> MDSTNLNKRPLLQYSLSSLGSQITKWSSSRPTSPVRKARSTENDFLSKQDTSSILPSINDDGGEQWYEKFKPNCLEQVAIHKRKLKDVQEALDAMFLPNAKHRILLLSGPSGCSKSTVIKELSKILVPKYRQNSNGTSFRSTPNEHKVTEFRGDCIVNDLPQMESFSEFLKGARYLVMSNLSLILIEDLPNVFHIDTRRRFQQLILQWLYSSEPLLPPLVICITECEIPENDNNYRKFGIDYTFSAETIMNKEILMHPRLKRIKFNPINSTLLKKHLKFICVQNMKMLKEKNKWNKRQEVIDYIAQETGDIRSAITTLQFWATSSGSLPISTRESTISYFHAIGKVIHGSHSTNNDNEMINNLFENSNNLLSKEDFKLGILENYNTFNKGE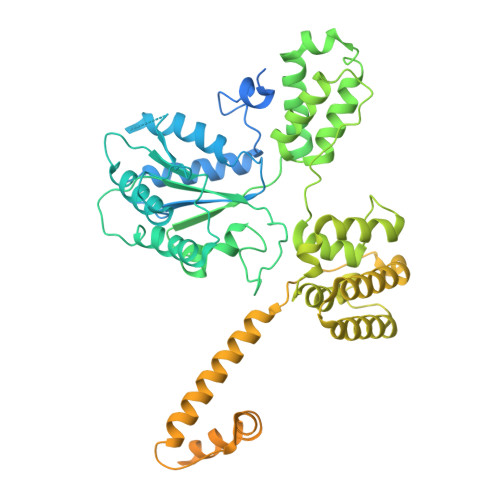FSISDASSIVDCLSECDNMNGLPESNEYGLREVRKTFRNISKQGHNHGTVYFPREWKVRKLQNSFKVQAEDWLNVSLYKYNAVHSFRNITLEFGYYAPLIRKCQSYKKKYILYYLKNLPSGSSGPKQTMDKFSDIMKVENGIDVVDRIGGPIEALSVEDGLAPLMDNDSNNCDHLEDQKKERDRRLRMLIDQYERNVMMANDDLEDEETSFNDDPIVDSDSDNSNNIGNETFGRSDEDESLCEILSQRQPRKAPVISESLSDSDLEIL> GSSVLSDLHEAVPTVVGIPDGTAVVGRSFRVTIPTDLIASSGDIIKVSAAGKEALPSWLHWDSQSHTLEGLPLDTDKGVHYISVSATRLGANGSHIPQTSSVFSIEVYPEDHSELQSVHTASPDPGEVVSSACAADEPVTVLTVILDADLTKMTPKQRIDLLHRM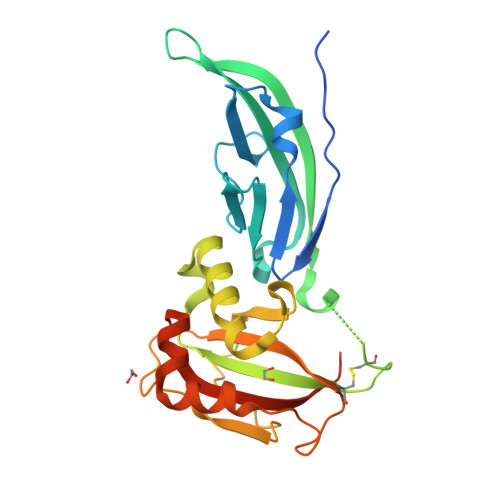RSFSEVELHNMKLVPVVNNRLFDMSAFMAGPGNAKKVVENGALLSWKLGCSLNQNSVPDIHGVEAPAREGAMSAQLGYPVVGWHIANKKPPLPKRVRRQIH>GPGHMDPDTFSYNFNNRPILSRRNTVWLCYEVERLDNGTWVKMDQHRGQVYSELKYHPEMRFLSLVSKWKLHRDQEYEVTWYISWSPCTKCARDMATFLQENTHVTLTIFVARLYYFWDPDYQEALRSLAQAGATIKIMNYDEFQHCWSKFVYSQGAPFQPWDGLDEYSQALSGMLGEILRHSMDPPTFTFNFNNEPWVRGRHETYLCYEVERMHNDTWVKLNQRRGFLANQAPHKHGFLEGRHAELCFLDVIPFWKLDLDQDYRVTCFTSWSPCFSCAQEMAKFISKNKHVSLCIKTARIYDDQGRAQEGLRTLAEAGAKISIMTYSEFKHCWDTFVDHQGAPFQPWDGLDEHSQDLSGRLRAILQNQEN[2x];>MGHHHHHHSQDPMENRWQVMIVWQVDRMRINTWKRLVKHHMYISRKAKDWFYRHHYESTNPKISSEVHIPLGDAKLVITTYWGLHTGERDWHLGQGVSIEWRKKRYSTQVDPDLADQLIHLHYFDEASEGSQIKPPLPSVRKLTEDRWNK[4x];>[4x]MPRVVPDQRSKFENEEFFRKLSRECEIKYTGFRDRPHEERQARFQNACRDGRSEIAFVATGTNLSLQFFPASWQGEQRQTPSREYVDLEREAGKVYLKAPMILNGVCVIWKGWIDLQRLDGMGCLEFDEERAQQEDALAQQAFEEARRRTREFEDR

HIV-1 hijacks a host ubiquitin ligase complex using a viral infectivity factor, Vif, to degrade the antiviral factor, APOBEC3G (A3G). A3G is a human, single-stranded DNA (ssDNA) deaminase that catalyzes fatal mutations in genomes of viruses such as HIV-1 [Reviewed in 6–9]. Here we show reconstitution of the A3G-Vif complex and subsequent A3G ubiquitination in vitro and report the cryo-EM structure of the A3G-Vif complex at 2.8 Å resolution using solubility-enhanced variants of A3G and Vif. In summary, our high-resolution cryo-EM structure of sA3G-VC-RNA20 revealed that Vif binds sA3G through interactions with ssRNA.

Our cryo-EM structures consistently showed that base rA7 of ssRNA is accommodated in a cavity formed by corresponding loops of sA3G NTD. In the asymmetric unit of this sA3G-VC-RNA20 structure, a single sA3G assembles with two VCs, named VCred and VCblue. The ligand, RNA20, participates in both interfaces sA3G-Vifred and sA3G-Vifblue. Specifically, we found two dinucleotides, rG6rA7 and rC17rA18, that were well defined in protein pockets of sA3G NTD and Vifblue, respectively. A binding pocket for rG6 is formed by W127 (NTD), F268, and K270 (CTD) of sA3G and H43 and Y44 of Vifred. In particular, atom N6 of base rA7 is within range to form bifurcated hydrogen bonds with carbonyl oxygens of both P25 and L123. Although the pocket size is large enough to accept a purine base, guanine atom O6 would be repelled by the carbonyl oxygens of P25 and L123, resulting in selective accommodation of adenine base. The cryo-EM map shows that the base rA18 is accommodated in a cavity formed by amino acids R17, T20, L24 and P162 to K168 of Vifblue including the PPLP motif. Intriguingly, only the two nucleotides, rA7 and rA18, participate in base-specific interactions with their protein binding partners.2-[(~{E})-(4-oxidanylidenebutanoylhydrazinylidene)methyl]benzoic 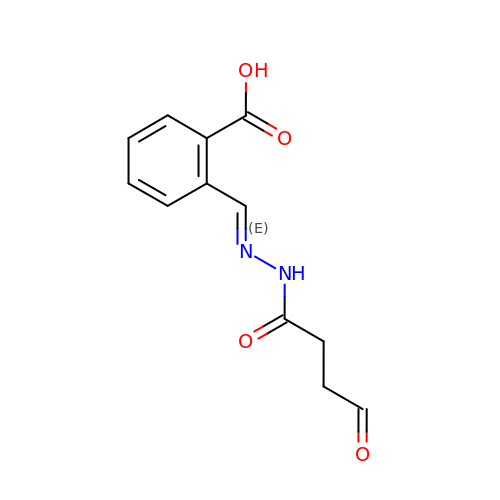acid | C12 H12 N2 O4 | OXKLPPJJEXEJQI-MDWZMJQESA-N>[2x]SIKTTRDRVPTYQYNMNFEKLGKCIIINNKNFDKVTGMGVRNGTDKDAEALFKCFRSLGFDVIVYNDCSCAKMQDLLKKASEEDHTNAACFACILLSHGEENVIYGKDGVTPIKDLTAHFRGDRCKTLLEKPKLFFIQAARGT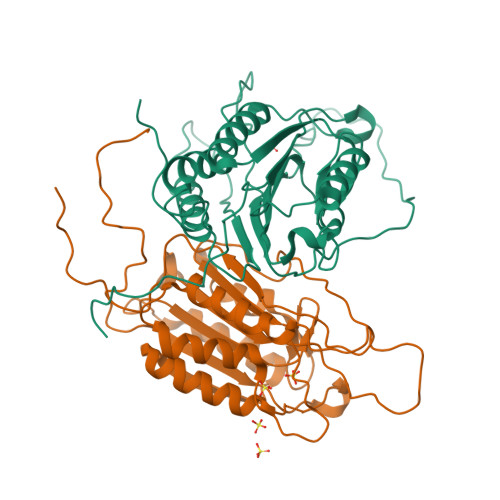ELDDGIQADSGPINDTDANPRYKIPVEADFLFAYSTVPGYYSWRSPGRGSWFVQALCSILEEHGKDLEIMQILTRVNDRVARHFESQSDDPHFHEKKQIPCVVSMLTKELYFSQLEHHHHHH Bacillus subtilis contains the SPβ prophage whose lysogenic state depends on the MrpR (YopR) protein, a key component of the lysis-lysogeny decision system. Structural characterization revealed that MrpR is a DNA-binding protein resembling the overall fold of tyrosine recombinases. MrpR has lost its recombinase function and the G136E exchange impairs its higher-order structure and DNA binding activity. MrpR functions as a master repressor of SPβ that binds to this conserved element to maintain lysogeny.

Crystals formed within one week of incubation, and we determined the structure of MrpR at a resolution of 2.9 Å by molecular replacement using the N-terminal domain (residues 1–105) of the MrpR Alphafold model and manually building the C-terminal part (residues 106–320). Two MrpR molecules were present in the crystallographic asymmetric unit. The monomers interact only weakly via residues of mainly two α-helices (helix H’ and I). As MrpR elutes as a monomer in analytical SEC experiments, the formation of a potential MrpR dimer appears to be an artifact of crystal packing. As other proteins with a tyrosine recombinase fold, MrpR harbors a CB (core-binding) domain (Gly1-Lys84, helix A–D) at the N-terminus, a catalytic (CAT) domain at the C-terminus (Tyr108-Ala320, helix F–M), which are connected by a central unfolded linker (Gly85-Leu107, helix/loop E). While amino acid sequence alignments of MrpR to tyrosine recombinases do not yield a high percentage of sequence identity (below 25 percent), structural comparison using PDBefold identifies the highest similarity to the structurally and functionally characterized tyrosine recombinases Cre from E. coli phage P1 (63,64), XerH from Helicobacter pylori, and the integrase (Int) from E. coli phage Lambda. Most of these tyrosine recombinases have been crystallized in complex with DNA to elucidate the recombination mechanisms in detail, while MrpR was crystallized in its apo form. While the CB domain in the MrpR crystal structure (in absence of DNA) is rotated by approximately 180° vertically and 45° horizontally compared to Cre, XerH and Lambda Int, the CAT domain needs to be flipped by 90° horizontally. We hypothesize that the observed organization of MrpR might be a crystallographic artifact since MrpR was not co-crystallized with DNA. The flexibility for the proposed rearrangements is provided by the approximately 22 residue-long linker present between the CB and CAT domain (labeled as helix E’ located between α-helices E and F), which is also present in Cre, XerH and Lambda Int. This structural rearrangement would also generate a positively charged groove between the CB and CAT domains of MrpR suitable for DNA interaction.

>[2x]MGHHHHHHMGFNSEIKEKYLDTLSEGMVMQMRPIFAKAEITETLYNKDIYDFTSMQILELIRSFDQTTIGSVRRTLALLSLYIDWAISYKLSKGLTNLARTISEEELYECLGDKKLYITYSELEEMENQLVNYQSKAVLRLLFEGVSGLAHSELLSLTKKQVEDAMLNGNVLTLYDSKHGERKLKVSSECLVIALNAAQETKYKLKNGKAKGQTKEVFLVENDYVVKTKRTSNKGDGQASKFVITNLITDISEFFKINFLTPNTIVRSGHLYRAYQLYKEKGVIDNSVRYQIIDDFNLRVKSKYRAVYSMQDYINEEEVNKYYAEELGLKETTILE>[6x]MNRVLYPGTFDPITKGHGDLIERASRLFDHVIIAVAASPKKNPLFSLEQRVALAQEVTKHLPNVEVVGFS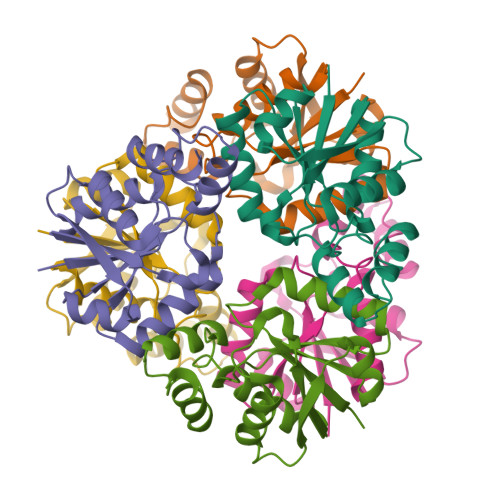TLLAHFVKEQKANVFLRGLRAVSDFEYEFQLANMNRQLAPDVESMFLTPSEKYSFISSTLVREIAALGGDISKFVHPAVADALAERFKR> MDKELDGRFERLEKALATMIDSLSKNNPSTKLAQDLVAAEAELLEGLKLLEAHQNNHARIQQLRQSTEQADAQIKDIISSLWKMRQELTSVQTSPIPKGAKFQFTTGELLDFARRISRNTLPPPGVTNGVNMTPAAARHSQQPSSVEPEDSFRVTSQSQTQTPNTSFNVSFNGTLVDTPGPFNNNSTPIPNAGPANSQNPHTELPEHLKLATNPLHGASFFPWPSVEQVRSGALGAYQLLVDKGIDPRGYDPEFEEQRRKDAEREAEERAKQEREEAERRAREEAERIARQRELERQRARESMAAAAEEGRRDSVVGGPAAGKPKQFTFLGGDDDDDDDDD;> MADPSSSTSAMPLDEIQWHTNPAVVGGSIHDNSVLFYFRESPFYDKTSNNEVLYQQGLHNQTMMQFLETRERFERRLREMSGLEFVVAQEPAETAPGTGTGVWVINKQTRRKRQGEEDEISVHGTYFLVGENVYMAAPTLADIISMRLASASSSISRLLPIAASVQSWSPGTGRVYKTPSMTSQTNQANQPSSQTQSQPTSQPATTTTTTALPPPDPRWLEETLMIHEFFGDHHLDKNPITGKPGDFHLSSTGRKIQTLPTAAAGNKKPGSGLPPLPAINTKVQQNPMGSGKQVTGKETKSPKTPSSSTGPGTGGMSTGMGKPKKRKSSKAAVTPTS;> MDSSEDDGNKVAHLWPDPPAFWKDFTPENIERYNALKQTYAQQHGLSSDALVRIPDVPADLINLQPPPEPVDGKWKLYGQQEALANSLQSLEDAGIQRLAPASETTSDSKHFDRGFELKKLAKSLLVNYLELMGIMSINPAHASEKVQDIKTIVLNFHHILNEYRPHQAREQLIQLMQDHLDAKRNETAAVRAVVDKAKRLIEGLASIEIPKVEDDNGRKAVEVERAALAERREIAAWQEADALFT;> MASLNLAPEELKQLELLRNRFAQLQSSLTSLAGNLIRTEPLPTYESLQASASILQQNLRSIQELMTENSDIFKRIAIHPSTNFPGRTQEHMLLQLLRKKLEPEVESWVEEARETARAAGIDVSKLSGPGGGAPTRGMNGYGDDDEYGLDDEDEGVPSDPFNEQWADMLETFQHSLHHYVTVQLKKQYTVEEQEMGIENVRTGLKRELGDEDEDEDEDEEEEEEGVAGVAGGAASQGAGAGTAGAAAKKPVIQPEYLFWLAARGDTRVSRNIEFEAMRKVAQTAKRPAPPR;> MTAPLPEGLTPDAVDTLTELSAIIKKLRAAQQQQAANPSSQAAAGGPGTTGAPGSQPSSSGPNATAAGGAIGTTSLPSSATTGPTPSNALHSVKELPATTDPIKHKLQRARAAVRLLGDMSRTMAQQEAELARLEERRRKQAAMLAKAQEE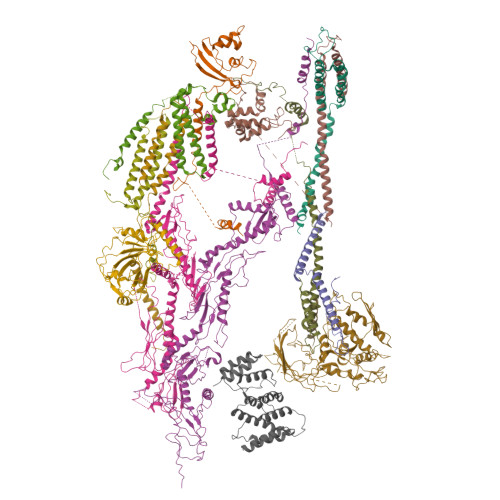GARLSKGFGEVGETPVVLVETGDKMAME;> MAQPSQSSVPESDAGSFPVDIHKPFTPAERIQQLGEIDNDIASLLQHLSAALKALATPPGKRIFQEQDSESNSPSASDTSNPNDTPPSSCGIDPVTAFKTAQNDFFRTIDRIDKHLTRQIYALEEAGIITLKSGTGSGAGTVGAGATEEQAQQLPQPQMIPGQPQAAGITADASVAPVPKARLEPDGMGRYGKLDVGRLNMASSIVEREMEGELWRKAREHLGRMTSQASGREDRMEE;> MEARAHGALPNNYDRERFINGVGGDDKALKRKLEEPLSDITKELDTVIAQSDVAVADPKGQLCPDADVPDEMEHITDGILPLNLLLIRLAEFSHSKLEELVTMLASKPVPQHAVNGNGSHSTLVEDASPESQEKKRLLLNTIQDLHSRWVKALVITEWARNAEKVGKLIDIRTHLFKKLELYPQVLNDFINLKRDMAWAKVPSPDLKTALHILTHGEVTWMPDFNFLDPPPLTTEETLRWINDMNLALHARLQLEEHDKLPPPFKNYTIDSGRVTFRVRGEFEVDLSISEEDFSEQFWFINFRFDFSPAPAELTPAVRYWMTEKVNNILKTEGLGGCYKYLHEFTLTQKIAELHRQAIALNKGRWANSLRVEKLNRNLGIHYWANRLHSQNLKSWIIIGVHSGEDPQGLEEPKPSYLMVQWFREGVEQFIDIPFSQEKLSIEEILEFVTAKHVGYLLFSLFRKFDGKPRFTQGKKARLELNVWTQKPEDYYLSMQLLDDEDLKIQVNPWMGDFITTPSTGPWNRTLNSLGNPAEEGSKELENFRYIYIISVLKAQGKSHGWSVVRSPISQDELRSIVHSESASSRETFQAAWTRFVDWDPQWYAMRSMSLAGDQWWLVEVTSQRQSISGNRLVFFTKMAPCFSEERLTDGFFNGLRDHSRRLIAEITNLRELYPGITPSQLRKLIDPTRQPPVLPVKASKILGDFGGADAQSIAWLKDPVWLIYRGSACDAAATRVSDSPQQKRTQPVLDVFEAYLDVTDRRRFQTLNPRLDRDILYNPYTGRFMFRLRAKMGVPVVPLLGIRVRQLQRLLDFLEGLRRVGDQAVPERVTLREIVFSYGATRKRDSTNQPKVRPWRVRLDLTKEEGVGVVLEKGNPHLRVINRLEDLVNSQKFYSLATYLTLSLPLFRAFEQLENAWQTAQENGRGSCFILHLSLDKHTIRFVLPGHQRQISLLIQPHEKEGKLVWEVGRPRHDPELLNENCEFNRVLKERVWTISGSGFKGLVTGAAAEPDEGIERLLVLISDAVLHLSTSQPATAPPQPPQAQPSQQVQQVQQQQVVSQLQPQAQQPRSAMPHASVGQQQPHGAPAPMARFPPQQQQIFQQQRPPQPQPNMHGGQISQPNMHGGPKPQLQGQHGQPGQMVAAPQQQGQRPGTGTAAGMGRSNAPLVVLD;> MTDRPFILQVPPTQQRGPQNIAEFVARINPDAFRVLNEAELRRKVEEEKNGVGQDEDVDMESSPSDNEGEPADAKDIITAKHEMLRVIDQTRQTTLYALDFVSLLLSKENPGQAVTTFSPGLRELVGIGTLGATMLDAPTPLTQSRIPDNKLVTIGKRLMDLNKAADTALAASKRLQKEIAAETKYWSEVLAVRNDGWQTSRMPREPQTMGVKFGFNNAAPEFKAVSIAPMRRADNGSVLLDRSSIGHKSQRIQVRILEDGRIVGRSSLPSPVSADAPLQDRVKEMRDTIFAQELWHEINREARTLLNQGVHLEPSSITYTMDASTTVSIRLATLGEEEEGLDEQQEGPQDVMAESLNIALSLLLSHAHRMNELRRSEPGINKGPPRTYPILLPLISYHKYNQSIQTCLQTLSAHISVLRSASVDSSMTVKEPLLSSPPGAPAATSLYTILTRPPAVQFDITITPDSRIRILLKPTQLTGAAFSICCLPALHPGAQNPLATTCPPSTDDYDSLTQVVSYLQAAIPRALAAHYEAVLVVEATVNGGMLGDLPPSPSRWMPLIDGKGIVDPETMRFGIRFSFGRNPAKGGQLELGAQTDYVDGSRKRVRRNWIWPGAQSSLDSVAKHVLARGPPEE;> MPYEIFLAGVVSDNDEAKARAVLGGFTEMREHHRFTRVQHYEPQDIKIRGFPTIKELLKERGPTTALYQELHNILVRQPYTLQIRTNITDAILGPAQAGAEAAPHGTVSGGKPHILRWSDIPDPPNQRIPPFITQRKIIEIPDQRAPRILAASKFRNKSDLVEESYHWWFNDVEYSMVRTYLISLDPSPQTTDQVPSLAGLEPIGDFWLLYVRMRVEATPDRMQQAHNQLQQIRDQLLGVFEFKVWDRRAHDTRIMEQPTQGNGNVIGDAHNSNKKSNGVSPTTASSSEEVSPVDSQLTIPLPDDDDGDNVEDTPDTEMDEDDDESEYDSDSERDWPKDD;> DRLTQLQEAMDELLEMFLSAFFWVERHHDLKTFGPNDKIPDLKADQPKEVDTKSPEEYKAGQLQLARDIIVKEQQIEYLISTLPGLDNSEREQIQLLRELEDDLVTAEAQRQEALKERDEVLGKLDALLRGLERP;> MDRDQGASDNLLERKNILIASIMTSYRDLITHATSPITSATASPGHAGYSSMALSTAIHAAVKYTEDLLSLTRTLREALWVVGPLTGPGEKDAQAEEGMAKDAEVVWDVLNEMRDRERERMMAALMEGDTRVRGAVRFERGDVEVVVAGQGQQIEMGRGVNGEVKSEGA;> MSVDSSGMEPPPLPSDGPEEPKHGGHTRFELELEFVQALSNPEYVNWLASRKYLMNPAFVAYLDYLQYWSRPPYLKYLTYPTATLRMLQLLQSERFRQEILVPDVAWQLRLEGMKAAVLWHKEG;> MSTPIPTPGRNPLQGRTPSQAHGAAGTPPVSTPFSAAQAVFSPNGPRSSPQQFKRSPATVGSTTATGGRPPSAINFDSPSASAALGALQPMTPGMDMTIRSLANLGRASEDERAKRLEEVIHILSKSKGLVSEAGLERLARSLELEFMWESSMGSDNKRTLIVAGSALELLVEFSQDVVQSVTLNFPDSPEIVTKHAQKAGEILFNDLRLAPGQSPLTKSLARFAANFERLAVLDKLSILPGLNLYEAVADVYESLARLHAWELQKLREDPSLAGKDDEYLENLVLCTKSGKPAMNDRGRVGLALDYWKEKHLLRTPEAEVASWIADNERTWSILIGCAPLRDLSINPVRISDKWIGPNVVKTSLPDGLHTGEPIIDWLDPEPTFIPATDQQQQQQQQQQQQQQQQQQQQQADAPLLPPRLPEVAFHAVFDPPVHIPINLWQHLQEMGCVLPDETATQPFQQHHFRSFDSLVIPPPQGKETDATETRVFSCRKKTPFVPRRSGVRNGEGATQKMEYRIHQNTLFVPKPVMCRTLTEMSFSHPQQLVSILPYLRQYAFLAQLLENSFKPGPALQLPTDPNADTTTSKPTPNAKASHKKLDDFEAFLAKHSSHSGPISNMTPSQHQPSSDLSIDVTLRLVLPSPKLQIVFPLHATSKEEVKGKIAHVTFAVRENGRLEVEMQNMIEEEGDQMEGVKTEGDEDGEEKKRRRPQPGDLARALEVLEDVGKWAEFVRTRWV>[2x]MSLNEEQLSKRLEKVASYITKNERIADIGSDHAYLPCFAVKNQ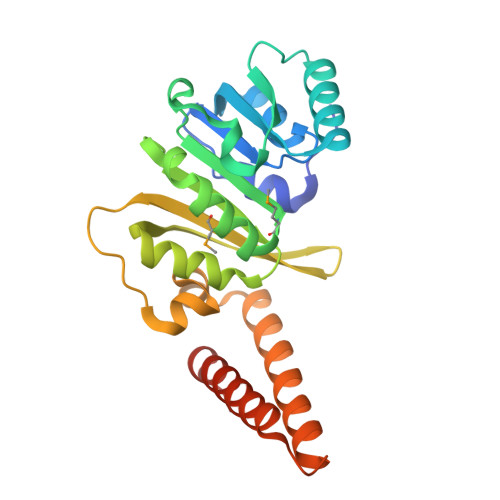TASFAIAGEVVDGPFQSAQKQVRSSGLTEQIDVRKGNGLAVIEKKDAIDTIVIAGMGGTLIRTILEEGAAKLAGVTKLILQPNIAAWQLREWSEQNNWLITSEAILREDNKVYEIMVLAPSEKPVTWTKQEIFFGPCLLKEQSAIFKSKWRHEANTWQNIIQTISNNQPVSTENQAKIRELEHKIALVEDVLKEGHHHHHH1-(3-chloranyl-4-methoxy-phenyl)-3-[7-[(3~{S})-3-(methoxymethyl)morpholin-4-yl]-2-methyl-pyrazolo[1,5-a]pyrimidin-6-yl]urea | C21 H25 Cl 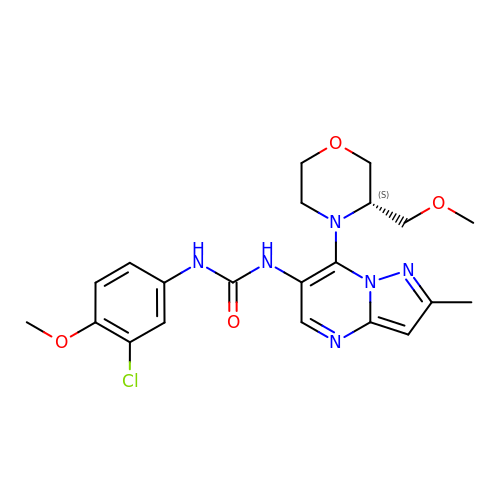N6 O4 | IUORVTKNCDNHNC-HNNXBMFYSA-N> GUGCGACAAGAAGUUCAGGAAGGGAUUGAGGUGAAAGUCCUCCUCCCGAAUCGUUCAUGGGAGAGUCUAUCCAGACUUGCGUAGCGAGUAAUCGCUAGGUGAGAAGCUCUGGAGACAAUGUACCUGCCCUUCAAUUGGAGGUGCCAGGGCUAGGCUUUGUUCCUAUGGCUAGCGAAAGCGAAUACAGGUUAUUAGGCGUCGUGAAAACAAAACUCUUUCGACAUAAGGGAGAGGCUCGUAGAUGAGUUACCCUCCUUUUUAUGGGGUAACUGAACGAUCAAUAUCUACCGGCGUAGACUGUGAGCCUAAAGGAAACGAAUGAAAGUGUCCCUUCCUGGGAACUUGGUAAGCCCAAUAGACUCCCUCUGGGAAACCAGAGGAGGAGUAAGAGCAAUCUUACUUAUCGUCUAGUGGGUAAAAGACAUAAUAGGAAGCAAAUGCUUGGUUGUAACGAUCGAGAUAGAAUCUGUUGAUUUAAGCUGAAAGGCUGCAGACUUAUUAAAUGGGUGUUCUGCUGUAUGGCGUUCGCGCCUAAGCAGCAGAAUGCGUGAGCCGUGUGCGAUGAAAGUCGCAAGCACGGUUCUGAUGGGGGGAAAACGAGAGAUCGUCUACCUAUCCAACU;> ACUGUUUAUUAAAAAC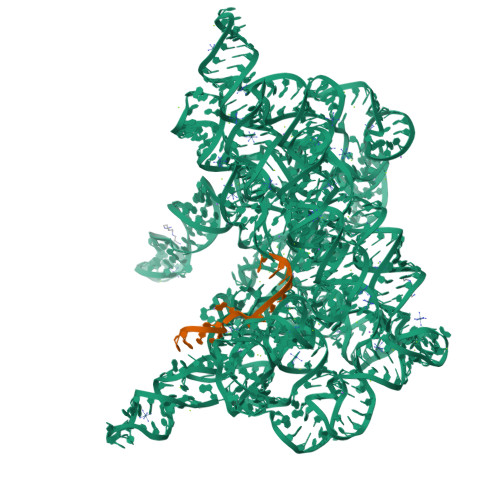ACAG> TYQYNMNFEKLGKCIIINNKNFDKVTGMGVRNGTDKDAEALFKCFRSLGFDVIVYNDCSCAKMQDLLKKASEEDHTNAACFACILLSHGEENVIYGKDGVTPIKDLTAHFRGDRCKTLLEKPKLFFIQACRGTELDDGIQADSGPINDTDANPRYKIPVEADFLFAYSTVPGYYSWRSPGRGSWFVQALCSILEEHGKDLEIMQI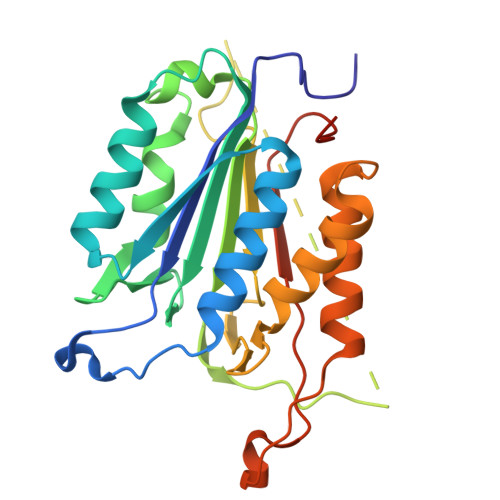LTRVNDRVARHFESQSDDPHFHEKKQIPCVVSMLTKELYFSQQLHHHHHH> MIAFQYLTATIMILLGIYALLYKRNLIKLVLALNLIDSGIHLLLISEGYRMENGIPPTAPIYTGYEGGAMVAPIPQALVLTSIVIGVCVLSL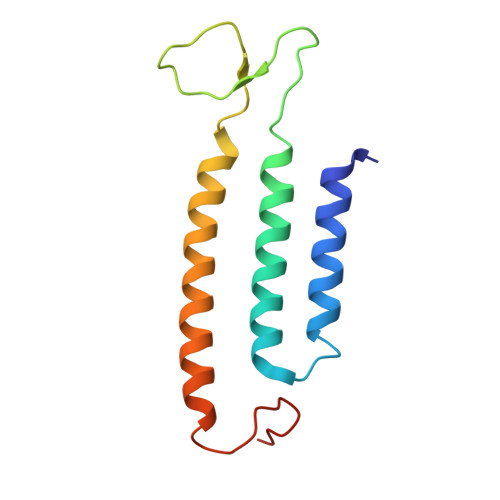AIALTVNAYRHYGTLDVTKLRRLRG> GLPVLNTPGSNQYLTADNYQSPCAIPEFDVTPPIDIPGEVRNMMELAEIDTMIPLNLTNQRKNTMDMYRVELNDAAHSDTPILCLSLSPASDPRLAHTMLGEILNYYTHWAGSLKFTFLFCGSMMATGKLLVSYAPPGAEAPKSRKEAMLGTHVIWDIGLQSSCTMVVPWI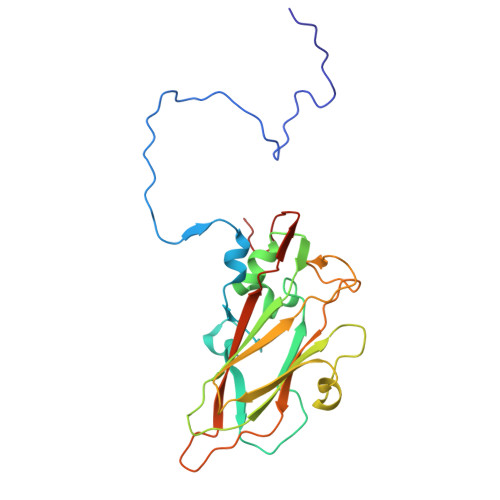SNTTYRLTINDSFTEGGYISMFYQTRVVVPLSTPRKMDILGFVSACNDFSVRLLRDTTHISQEAMPQ D,L-Propargylglycine (PAG) has been widely used as a selective inhibitor to investigate the biological functions of cystathionine γ-lyase (CSE), which catalyzes the formation of reactive sulfur species (RSS). CSE produces H2S during the metabolism of cysteine, and also generates cysteine persulfide (CysSSH) from cystine as a substrate. However, PAG also inhibits other PLP (pyridoxal-5′-phosphate)-dependent enzymes such as methionine γ-lyase (MGL) and L-alanine transaminase (ALT), so highly selective CSE inhibitors are still required. Here, we performed high-throughput screening (HTS) of a large chemical library and identified oxamic hydrazide 1 as a potent inhibitor of CSE (IC50 = 13 ± 1 μM (mean ± S.E.)) with high selectivity over other PLP-dependent enzymes and RSS-generating enzymes.

We then determined the high-resolution (1.9 Å) X-ray crystal structure of the rCSE complex with 1, and found that the hydrazide group of 1 forms a Schiff base linkage with the aldehyde group of PLP in the active site of rCSE, affording PLP-1. Moreover, several amino acid residues of rCSE (Glu339, Ser340, Arg375 and Asn161) around the CSE active site form hydrogen bonds with oxygen atoms of 1 in PLP-1. These results are consistent with the observed strong binding of 1 to rCSE in the SPR measurement. The optimized cis form showed a dihedral angle defined by N–C–C–N of the dicarbonyl structure of PLP-1 of around 40 degrees, while the energy minimum of the trans form was located near the dihedral angle of 180 degrees. These results indicate that PLP-1 can take both cis and trans conformations, though the cis-form of PLP-1 appears to be preferred in the crystal structure as judged from B-factor analysis. In this context, it is noteworthy that the substrate pocket of rCSE is relatively small in our X-ray crystal structure. In the pocket of rCSE, PLP occupies 181 Å3, while the size of 1 is 71 Å3. In addition, PLP is located at a position that restricts entry to the pocket, and it is estimated that the space through which molecules can enter is only about 70 Å3. Thus, the covalent bond formation between 1 and PLP seems likely to contribute to the high selectivity and potent inhibitory activity of 1 toward CSE, in addition to the multiple hydrogen bonding interactions between the inhibitor and the amino acid residues at the active site of CSE. We also confirmed that all amino acid residues of rCSE involved in the recognition of 1 are conserved in hCSE.

>[12x]GPGFLPSFQHFATQAIHVGQEPEQWSSRAVVLPISLATTFKQDSPGQSSGFVYSRSGNPTRNCLEKAVAALDGAKHCLTFASGLAATTTITHLLKAGDEVICMDEVYGGTNRYFRRVASEFGLKISFVDCSKTKLLEAAITPQTKLVWIETPTNPTLKLADIKACAQIVHKHKDIILVVDNTFMSAYFQRPLALGADICMCSATKYMNGHSDVVMGLVSVNSDDLNERLRFLQNSLGAVPSPFDCYLCCRGLKTLQIRMEKHFRNGMAVARFLESNPRVEKVIYPGLPSHPQHELAKRQCTGCPGMVSFYIKGTLQHAQVFLKNIKLFALAESLGGYESLAELPAIMTHASVPEKDRATLGISDTLIRLSVGLEDEKDLLEDLGQALKAAHP> RLLEDALIAVRQQTAMMRKFLDTPGKLMDALKCCSTLVSELRTSSLSPKQYYELYMAVFDALRYLSAHLRENHPVNHLADLYELVQYAGNIIPRLYLMITVGTAYMSIDGAPVKELMK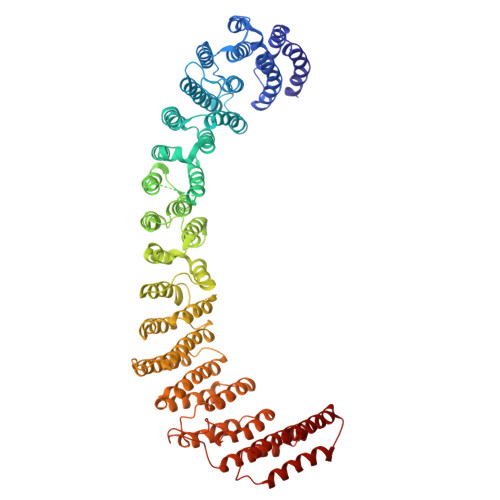DMMDMSRGVQHPVRGLFLRYYLSGQARDYLPTGDSDGPEGNLQDSINFILTNFVEMNKLWVRLQHQGHSRERDLRTQERRELQLLVGSNIVRLSQLVDLPTYRDSILGPLLEQIVQCRDILAQEYLLEVITQVFPDEYHLHTLDQFLGAVSRLNPHVNVKAIVIGMMNRLSDYAERESQNEPEEDRAKLEEEALAKLLEKTKLGQNSELEPQNGDHPDTEVSSTTDSAQAPSTADSDTTAVNGEEEPVRKRRGIPVNVPLYDIFFDQVQHLVQAQHLPIQDTIALCCSLANLSLNIYPERLDYVDGILAYALAKVKEHANSADLHSQPAQQSLLSLLQSPLRRYVSIFTALSLPTYVSLFQAQTYPTRRAIAGEIVRTLLKNQTLISTPAHLENVLEILKVLIKEGSQPPAGYPGVVQPRARPLETDETMEEQGWLARLVHLIHSDDNDTQFRLLQMTRKAYAEGNERIRTTTPPLITAGLKLARRFKAREHYDDNWSSQSSSLFKFLHSAISTLYTRVNGPGVADLCLRLFCSCGQVADMTEFEEVAYEFFAQAFTVYEESISDSKAQFQAVCVIASALHRTRNFGRENYDTLITKCAQHASKLLRKPDQCRAVYLASHLWWATPIAARGETEDTELYRDGKRVLECLQRALRVADSCMETATSIELFVEILDRYVYYFDQRNESVTTKYLNGLIELIHSNLAGNQQDSASVEASRKHFIQTLEMIQ> SLQTVLVNRMVELATGPELGAMDLLFDEFRAAHVPVEEMATHYIPEAARQIGAAWDSDRIGFAQVTIAISRLQELLHALQTLVTADSVGCANGATVLLIVPPGEQHTLGALIVAMELRRRGVSVRIVFAPGLSDLSRLMATTRFDAALITVGSMDRVEICAKLVKTLSSLTKG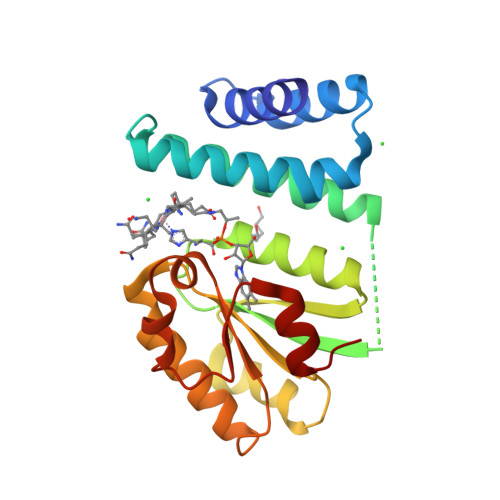RMRVAIGGAIVSQRAEALARTGADLVTNDLSLVISEFSLV> MEAGITGTWYNQLGSTFIVTAGADGALTGTYVTARGNAESRYVLTGRYDSAPATDGSGTALGWTVAWKNNYRNAHSATTWSGQYVGGAEARINTQWLLTSGTTEH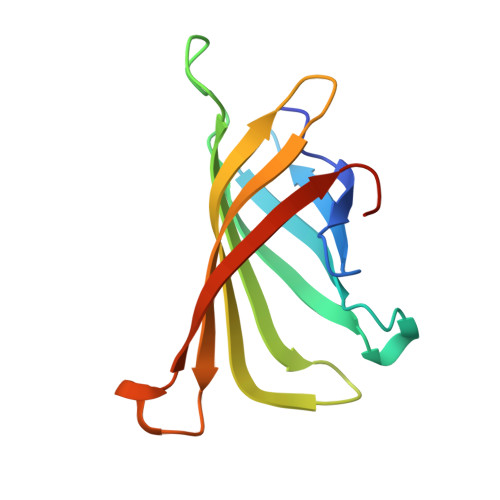WYSTLVGHDTFTKVKPSAAS> QAQITGRPEWIWLALGTALMGLGTLYFLVKGMGVSDPDAKKFYAITTLVPAIAFTMYLSMLLGYGLTMVPFGGEQNPIYWARYADWLFTTPLLLLNLALLVDADQGTILALVGADGIMIGTGLVGALTKVYSYR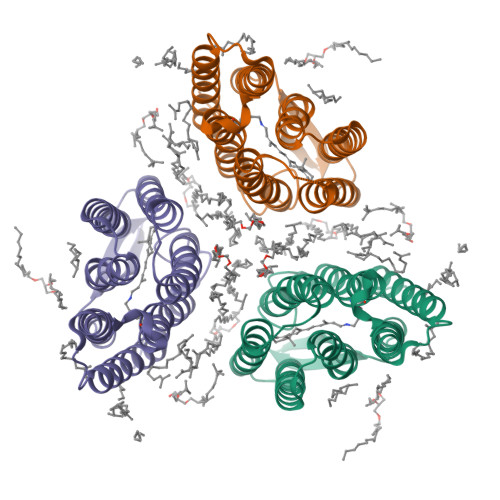FVWWAISTAAMLYILYVLFFGFTSKAESMRPEVASTFKVLRNVTVVLWSAYPVVWLIGSEGAGIVPLNIETLLFMVLDVSAKVGFGLILLRSRAIFGEAEAPEPSAGDGAAATSD> GDAWQDDEYFGNYGTLRLHLEMLSDKPRTETYRQVILSNSAALREKVVLDLGCGTGVISLFCALLAKPAGVYAVEASSMAEHTEELVKQNGCDGVVTVFQERAENLTLPTKVDVLVSEWMGNCLLFEYMLESVLLARDRWLKKGGMMWPSSACL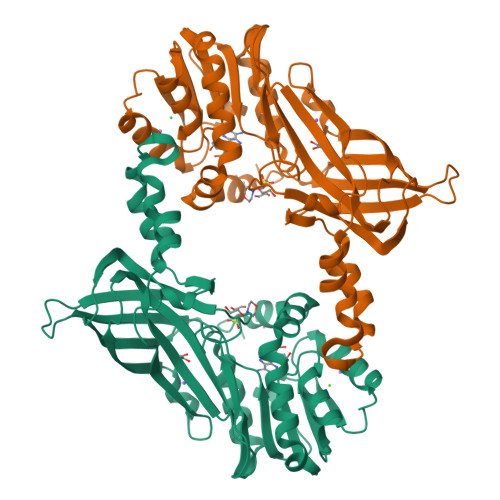TIVPCQAFSDYRQKVEFWENPYGLNFSYLQSLAQKEFLSKPKFSHHLQPEDCLSTPADVITLDMVTIQVSDLERLKGEFTFTVEKSGMFHGFTVWFSAHFQCLEEDGPSIELNTGPYSEITHWKQTLFMLDAPVSVEEGDIIAGSIRLQRNPIWRRHLSITFLWNINSTEVSTVKTKCFPMWR> MAHHHHHMFRIVVGLGKSGMSLVRYLARRGLPFAVVDTRENPPELATLRAQYPQVEVRCGELDAEFLCSARELYVSPGLSLRTPALVQAAAKGVRISGDIDLFAREAKAPIVAITGSNAKSTVTTLVGEMAVAADKRVAVGGNLGTPALDLLADDIELY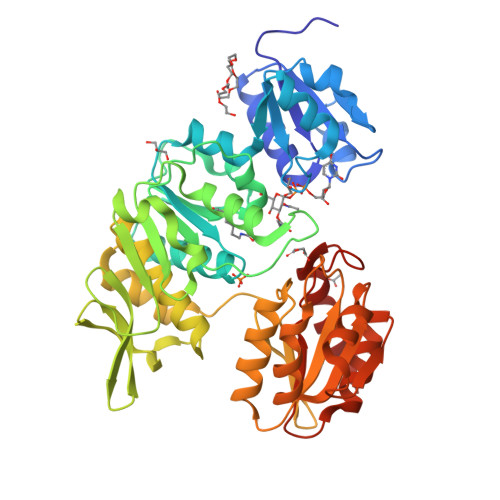VLELSSFQLETCDRLNAEVATVLNVSEDHMDRYDGMADYHLAKHRIFRGARQVVVNRADALTRPLIADTVPCWSFGLNKPDFKAFGLIEEDGQKWLAFQFDKLLPVGELKIRGAHNYSNALAALALGHAVGLPFDAMLGALKAFSGLAHRCQWVRERQGVSYYDDSKATNVGAALAAIEGLGADIDGKLVLLAGGDGKGADFHDLREPVARFCRAVVLLGRDAGLIAQALGNAVPLVRVATLDEAVRQAAELAREGDAVLLSPACASLDMFKNFEERGRLFAKAVEELA>[2x]STAGKVIKCKAAVLWEEKKPFSIEEVEVAPPKAHEVRIKMVATGICRSDDQVVSGTLVTPLPVIAGHEAAGIVESIGEGVTTVRPGDKVIPLFTPQCGKCRVCKHPEGN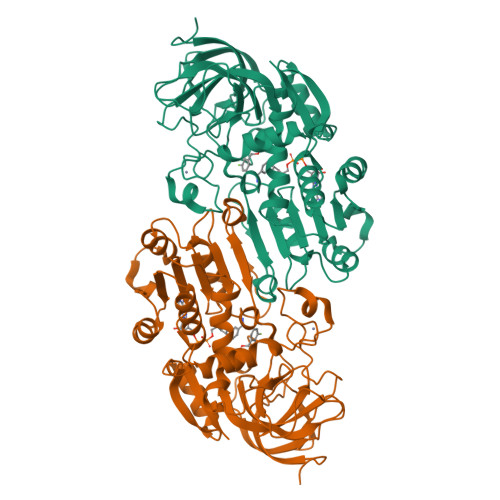FCLKNDLSMPRGTMQDGTSRFTCRGKPIHHFLGTSTFSQYTVVDEISVAKIDAASPLEKVCLIGCGFSTGYGSAVKVAKVTQGSTCAVFGLGGVGLSVIMGCKAAGAARIIGVDINKDRFAKAKEVGATECVNPQDYKKPIQEVLTEMSNGGVDFSFEVIGRLDTMVTALSCCQEAYGVSVIVGVPPDSQNLSMNPMLLLSGRTWKGAIFGGFKSKDSVPKLVADFMAKKFALDPLITHVLPFEKINEGFDLLRSGESIRTILTF> GSSMGSQSLYREIHQLISFKDVLPDKNLLPDWSSNKNPCTFDGVTCRDDKVTSIDLSSKPLNVGFSAVSSSLLSLTGLESLFLSNSHINGSVSGFKCSASLTSLDLSRNSLSGPVTTLTSLGSCSGLKFLNVSSNTLDFPGKVSGGLKLNSLEVLDLSANSISGANVVGWVLSDGCGELKHLAISGNKISGDVDVSRCVNLEFLDVSSNNFSTGIPFLGDCSALQHLDISGNKLSGDFSRAISTCTELKLLNISSNQFVGPIPPLPLKSLQYLSLAENKFTGEIPDFLSGACDTLTGLDLSGNHFYGAVPPFFGSCSLLESLALSSNNFSGELPMDTLLKMRGLKVLDLSFNEFSGELPESLTNLSASLLTLDLSSNNFSGPILPNLCQNPKNTLQELYLQNNGFTGKIPPTLSNCSELVSLHLSFNYLSGTIPSSLGSLSKLRDLKLWLNMLEGEIPQELMYVKTLETLILDFNDLTGEIPSGLSNCTNLNWISLSNNRLTGEIPKWIGRLENLAILKLSNNSFSGNIPAELGDCRSLIWLDLNTNLFNGTIPAAMFKQSGKIAANFIAGKRYVYIKNDGMKKECHGAGNLLEFQGIRSEQLNRLSTRNPCNITSRVYEGHTSPTFDNNGSMMFLDMSYNMLSGYIPKEIGSMPY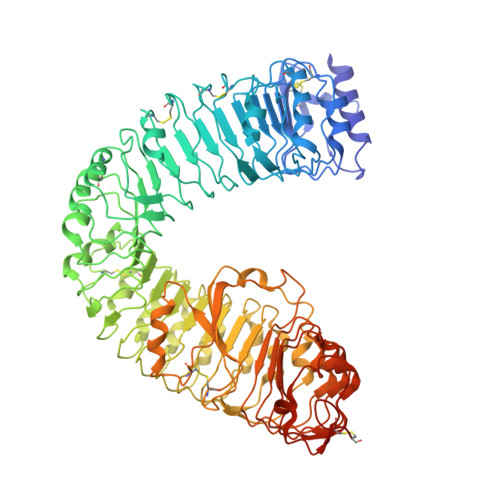LFILNLGHNDISGSIPDEVGDLRGLNILDLSSNKLDGRIPQAMSALTMLTEIDLSNNNLSGPIPEMGQFETFPPAKFLNNPGLCGYPLPRCDPSNADGYAHHQRSHGRRLENLYFQGA>KDDFAKLEEQFDAKLGIFALDTGTNRTVAYRPDERFAFASTIKALTVGVLLQQKSIEDLNQRITYTRDDLVNYNPITEKHVDTGMTLKELADASLRY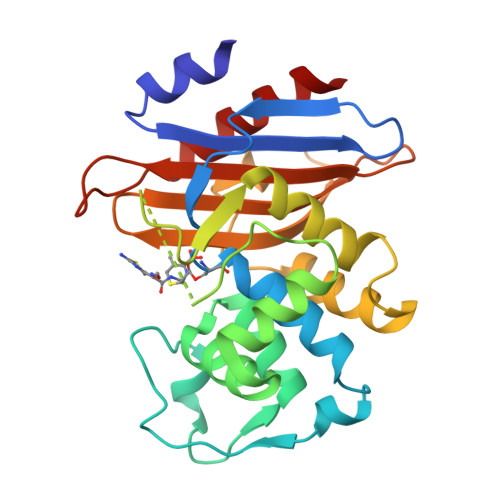SDNAAQNLILKQIGGPESLKKELRKIGDEVTNPERFCPELNEVNPGETQDTSTARALVTSLRAFALEDKLPSEKRELLIDWMKRNTTGDALIRAGVPDGWEVADKTGAASYGTRNDIAIIWPPKGDPVVLAVLSSRDKKDAKYDDKLIAEATKVVMKALN[2x]>[2x]MGSLVNRKQLEKMANVRFRTQEDEYVAILDALEEYHNMSENTVVEKYLKLKDINSLTDIYIDTYKKSGRNKALKKFKEYLVTEVLELKNNNLTPVEKNLHFVWIGGQINDTAINYINQWKDVNSDYNVNVFYDSNAFLINTLKKTVVESAINDTLESFRENLNDPRFDYNKFFRKRMEIIYDKQKNFINYYKAQREENPELIIDDIVKTYLSNEYSKEIDELNTYIEESLNKITQNSGNDVRNFEEFKNGESFNLYEQELVERWNLAAASDILRISALKEIGGMYLDVDMLPGIQPDLFESIEKPSSVTVDFWEMTKLEAIMKYKEYIPEYTSEHFDMLDEEVQSSFESVLASKSDKSEIFSSLGDMEASPLEVKIAFNSKGIINQGLISVKDSYCSNLIVKQIENRYKILNNSLNPAISEDNDFNTTTNTFIDSIMAEANADNGRFMMELGKYLRVGFFPDVKTTINLSGPEAYAA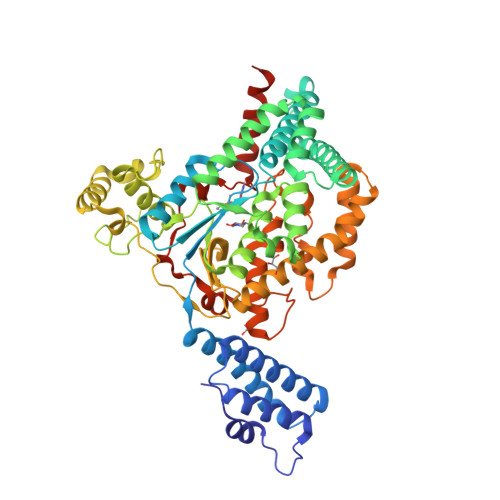AYQDLLMFKEGSMNIHLIEADLRNFEISKTNISQSTEQEMASLWSFDDARAKAQFEEYKRNYFEGSLLEHHHHHH>[2x]SNAKVILYARVSSN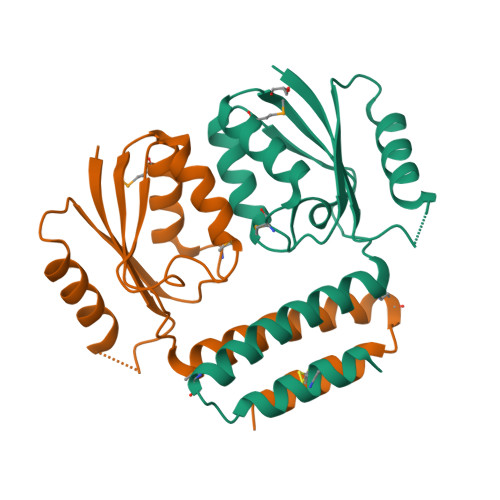TQKDDLANQVKYLEEQVKEYDLVITDIGSGLNMKRKGFLKLLRMILNNEVSRVITAYPDRLVRFGFEILEEVCKAHNCEIVVLNQEDKTPEEELVEDLATILVSFSGKLHGMRSQKYEKVKKCAEELKN N-{3-[4-(dimethylamino)piperidin-1-yl]phenyl}-4-fluoro-7-methyl-1H-indole-2-carboxamide 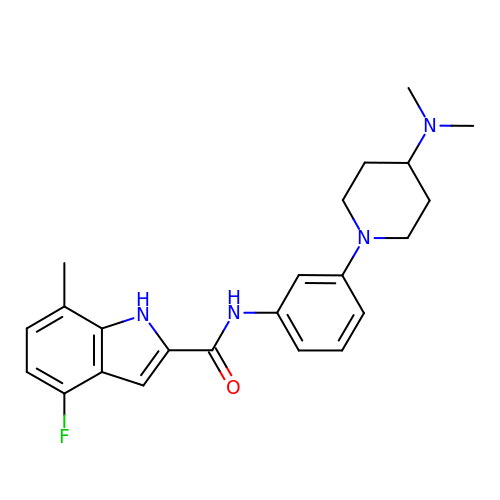| C23 H27 F N4 O | GBIAQCRLFDZGOQ-UHFFFAOYSA-N> MADEALFLLLHNEMVSGVYKSAEQGEVENGRCITKLENMGFRVGQGLIERFTKDTARFKDELDIMKF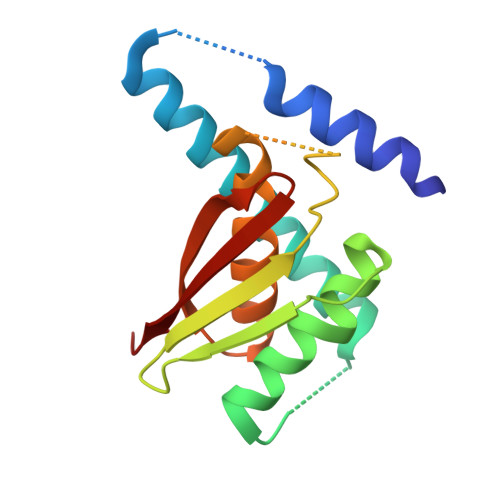ICKDFWTTVFKKQIDNLRTNHQGIYVLQDNKFRLLTQMSAGKQYLEHASKYLAFTCGLIRGGLSNLGIKSIVTAEVSSMPACKFQVMIQKL>GSHMELTPDQQTLLHFIMDSYNKQRMPQEITNKILKEAFSAEENFLILTEMATNHVQVLVEFTKKLPGFQTLDHEDQIALLKGSAVEAMFLRSAEIFNKKLPSGHSDLLEARIRNSGISDEYITPMFSFYKSIGELKMTQEEYALLTAIVILSPDRQYIKDREAVEKLQEPLLDVLQKLCKIHQPENPQHFACLLGRLTELRTFNHHHAEMLMSWRV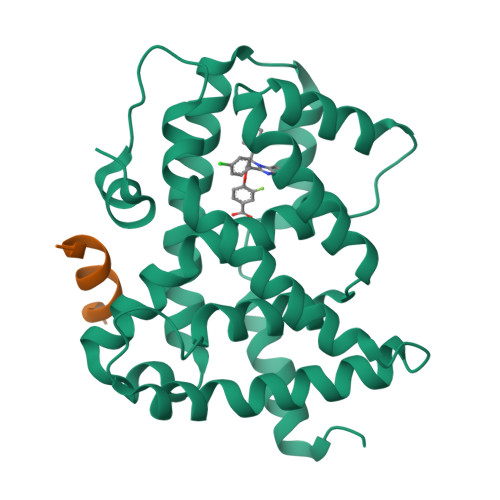NDHKFTPLLCEIWDVQ[2x];>KDHQLLRYLLDKDE[2x]> MEAIIISGTEMAKHIQKEIQR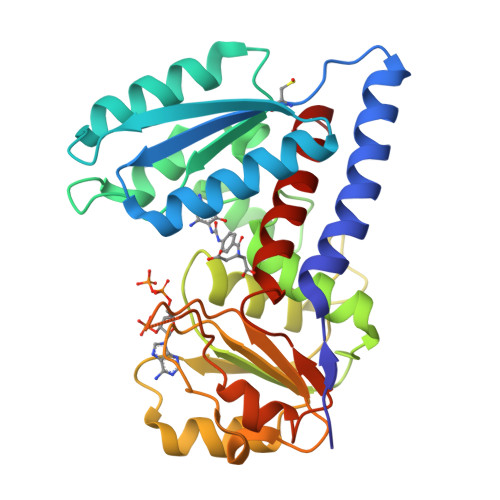GVESWVSLGNRRPHLSIILVGDNPASHTYVRNKIRAASAVGICSELILKPKDVSQEELLDVTDQLNMDPRVSGILVQLPLPDHVDERTICNGIAPEKDVDGFHIINIGRLCLDQHSLIPATASAVWEIIKRTGIQTFGKNVVVAGRSKNVGMPIAMLLHTDGEHERPGGDATVTIAHRYTPKEQLKIHTQLADIIIVAAGIPKLITSDMVKEGAAVIDVGINYVHDPVTGKTKLVGDVDFEAVKKKAGFITPVPGGVGPMTVAMLLKNTLLAAKKIIY> SMADCQGWLYKKKEKGSFLSNKWKKFWVILKGSSLYWYSNQMAEKADGFVN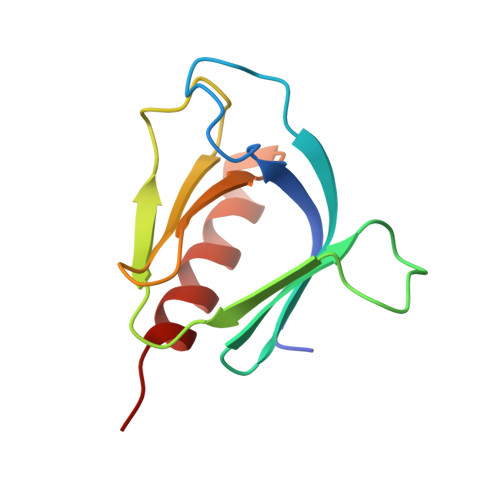LPDFTVERASECKKKHAFKISHPQIKTFYFAAENVQEMNVWLNKLGSAVIHQ>[4x]SNAMMDNMQTEAQPTRTRILNAAREIFSENGFHSASMKAI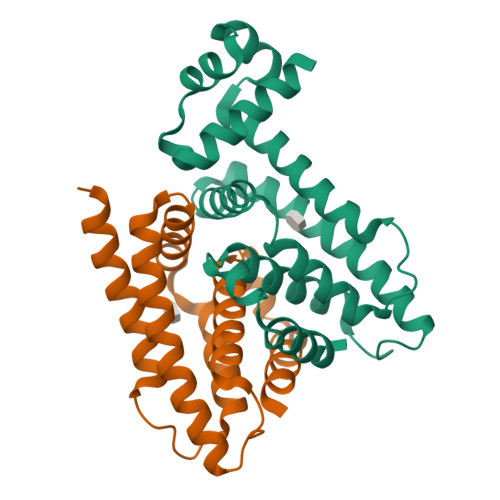CKSCAISPGTLYHHFISKEALIQAIILQDQERALARFREPIEGIHFVDYMVESIVSLTHEAFGQRALVVEIMAEGMRNPQVAAMLKNKHMTITEFVAQRMRDAQQKGEISPDINTAMTSRLLLDLTYGVLADIEAEDLAREASFAQGLRAMIGGILTAS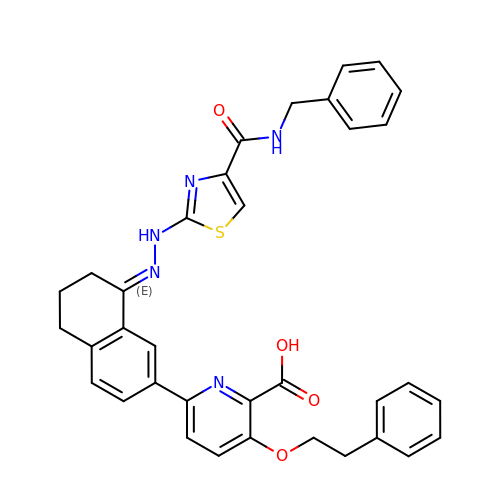6-[(8E)-8-{2-[4-(benzylcarbamoyl)-1,3-thiazol-2-yl]hydrazinylidene}-5,6,7,8-tetrahydronaphthalen-2-yl]-3-(2-phenylethoxy)pyridine-2-carboxylic acid | C35 H31 N5 O4 S | LPGFMHLHQPZQLK-YWIBTEMISA-N>[2x]RKPKTGILMLNMGGPETLGDVHDFLLRLFLDRDLMTLPIQNKLAPFIAKRLTPKIQEQYRRIGGGSPIKIWTS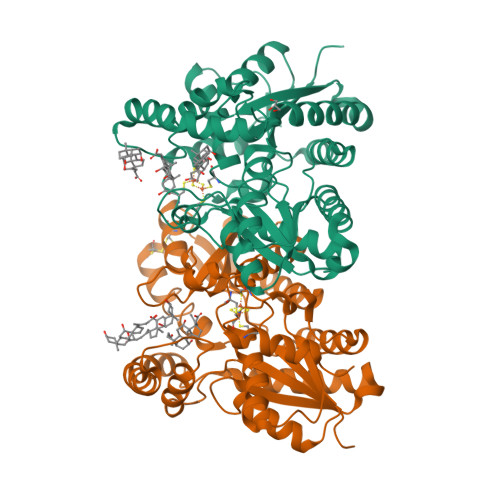KQGEGMVKLLDELSPNTAPHKYYIGFRYVHPLTEEAIEEMERDGLERAIAFTQYPQYSCSTTGSSLNAIYRYYNQVGRKPTMKWSTIDRWPTHHLLIQCFADAILKELDHFPLEKRSEVVILFSAHSLPMSVVNRGDPYPQEVSATVQKVMERLEYCNPYRLVWQSKVGPMPWLGPQTDESIKGLCERGRKNILLVPIAFTSDHIETLYELDIEYSQVLAKECGVENIRRAESLNGNPLFSKALADLVHSHIQSNELCSKQLTLSCPLCVNPVCRETKSFFTSQQL>MGSSHHSSGLVPRGSHMMSKTADAPGQTDVIVVGNGVLGLSVGVEIARTRPDVRVTLLGKPARQYGATPAAGAMLGAFGEVTAHALASEHGRKKHALAVQAQRLWPEWIESLEATGTAADGRIKTADDTVVLLNTVGHSALDDANFAAVLTALKEANAPHEEIAVESVDWIDPDPNSRPLRALHIEGEGSVDSGILLAALERSFLQAGGRLHPVDATEIRASHGRVEGVVTDDGDFLPAGHVVVAAGARSQRLVAALPGLAHRIPRIYDGVGVSALVDTWDGSGPATVLRTSNRAFACGLHLVPRAGGSVYIGATNAVCLEPRGAASIEETVALFNCATHQLHRGLNGSELRKVQVGSRPAPIDGFPLIGGTSVEGLWMLSGTYRDGLHMSPLLARHVVSLMDGGTGVDGLREFRPERDLISAWSREEILDDVVRHTMATGYEFPWRLPLEWPHMMETFLQGPFAELADRLSDTYTPPADLMTAIMFSEREQQDELIAYYADVHREWH[8x]

Here, we report a noncanonical FAD-dependent enzyme Orf1 that adds a glycine-derived N-formimidoyl group to glycinothricin to form the antibiotic BD-12. X-ray crystallography was used to investigate this complex enzymatic process, which showed Orf1 has two substrate-binding sites that sit 13.5 Å apart unlike canonical FAD-dependent oxidoreductases. One site could accommodate glycine and the other glycinothricin or glycylthricin. The resultant product is no longer sensitive to aminoglycoside-modifying enzymes, a strategy that antibiotic-producing species employ to counter drug resistance in competing species.

The residues nearby the C281-adduct include T298, E312, E313, F316 and E426, of which F316, E312 and E313 may cooperatively allow nucleophilic addition and cofactor-free decarboxylation reactions to proceed in sequence. Our reasoning is that F316 stabilizes the planar imine glycine adduct through the π-π stacking interaction. The importance of this residue was ascertained by mutational experiments, whereby F316A brings on 6 as the major product (Fig. 2a (vi)). On the other hand, superposition of the F316A-ST-F and C281-adduct complex displays that the long side chain of ST-F is subject to a geographic effect, resulting in flipping of the amide group away from E312 to accommodate the entire aliphatic sidechain. This posture is somewhat unexpected as the ε-amine of the β-lysine is a bit extended away from the α-carbon of the oximinoacetate adduct likely due to the absence of the phenyl ring (F316A). E312 not only recognizes the streptolidine base but also ushers the β-lysine to crawl into the binding site in a compact manner. In this context, E312A is able to catalyze the formation of 5 and 6 but no more 8, as opposed to F316A, which catalyzes the formation of 8, the dominant product (Fig. 2a (v), d (ix, x)). The enzymatic reactions in the presence of ST-F (compound 7) alongside glycine or isotopically labeled glycine suggested that the product is N-iminoacetyl-ST-F (compound 8). On the other hand, given ST-F the reaction gives rise to N-iminoacetyl glycinthricin, where the terminal carboxylic group is retained and the N–O bond undergoes dehydration afterwards.>[2x]MLTIGVLGLQGAVREH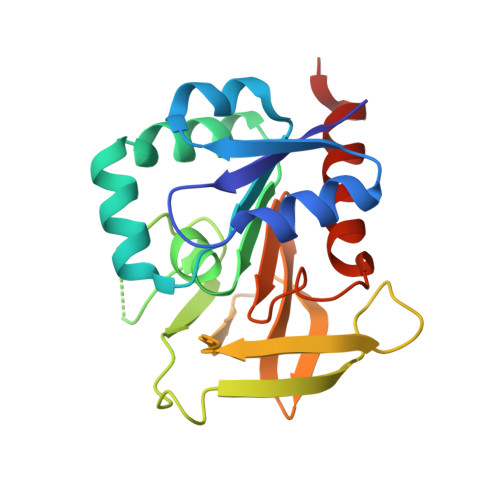IHAIEACGAAGLVVKRPEQLNEVDGLILPGGESTTMRRLIDTYQFMEPLREFAAQGKPMFGTCAGLIILAKEIAGSDNPHLGLLNVVVERNSFGRQVDSFEADLTIKGLDEPFTGVFIRAPHILEAGENVEVLSEHNGRIVAAKQGQFLGCSFHPELTEDHRVTQLFVEMVEEYKQKALV>MEEASSISRYLYTFIVLFIIWLFLTASLDPQELTIGALFSAIAALFTYEIFTTRGLANLHPKRVLYFIAYIPYFLWAMIMANLDVAYRVLHPKRPINPGIVECKTTLTNNVGKMALANSITLTPGTITLDVDGDKYFIHWIDVKDSSVEGASEHITKPFEKFLRVIFE[2x];>[2x]MIGVNIYLLLIGVATLLSMYRVFRGPTTVDRLVAVDIMTTITVGLMVLFALYYRRIIFLDVALVYAILSFAGVIAFARYLEGGL;>[2x]MSVLSLIGELLVLFGTVFYLLSTLGLIRMPDVYNRMQTATKSATLGSLGVIIGTGIWALGEGFSVAWLTKAIVIAAFLLLTNPISAHALIRAAYKSGIPLWEGSVVDKYKEHLERKKKEEGEQE;>MNCIVCIEYIIVALMIISAILAVEWRDLLASTVGMAAVSLFASILFFFLQAPDVAMTEAAIGAALSAAVFIFAIKRTYRYETEEEEKLGWWVRW[2x];>[2x]MLKRVLAILTILVIGYWLAQGLADVPFGQDKMVVGKYYLEHVKEETGAVNAVTAVVVNYRGLDTLGEVTVLFIASTGVAALLWKKKRERTAKTEGSVVLTTGARLLFPFIALFGMYIFIHGHLTPGGGFPGGATIATAFLLMYLAFTIYEIPHRGFEVTEGLAGMGYVITGLIGLAIGGYFLFDWIWQTWGWGHENIGRLFSGGFIPIIYTLIGIKVGTELSGIVDNMLKEEVKE;>MISSYYFGAISLILIGLYAVLVKKNLLKILIGLSIMETGVNLLLISIGYVSGKSAPILSEGVTASNAVDPIPQALVLTAIVIGVATTAMALSVAILLYEKYGTLNIEEIRRLRG[2x];>MSQVAALLIALPLISAFFVPVLKQIGKSLIKPFLVIITLLQTLIASWAFVQVYSTGKPIIIYAGGWKPPIGINLYIGHFAALFILVIAVVSFLMALFNFKAVTVEPIDKYAMLFLLLLLGATGMIATGDIFNLFVFMEITAISAYALTAYNKTGEAAEASMKYIVLGGIGSSFFLVGVALIYGATGTLNMAHLAMLANDINPTVVQVGLALIIFGLAVEAELFPLNAWAPDAYQAAPHPITVMFSAFVVKAGLYAMARILYLFKDVSGWSSLTKLLIAMATLTVVFAELSALRQKNVKRMIAYSSIGQVGLIALALSLGTQEGVSAGVFHMLNHAIVKTMMFMAIGYVGITLGGTMIENFEGLGKRMPLTSLSLTIGGIATVGVPLFNVFWSKLRIILAAAHEGNLWPVALVLFASVVEAVYYFRLIHTMWFKGKSGERIPEGAIAIVLLLLAMLIIVIGVYPTPFWNLVTKAGSDIVEVSKYVANVLPGVKL[2x];>MVDWRLFEPLFNWARKKSLWIVAFCTGCGGIEMPPLMTARYDLERFGIMPDPSPRQYDLFLITGYVTPKTLKRIIITYEMAPDPKYVLAHGSCPINGGIYWDAYNAIKQLDKYIPVDVYIAGCMPRPEAVMDGIKKLMEMIENGEADGWKRYKENYEWYRKNQDELLGEGWREKEARKWIPWLMDKRKEVKE[2x];>[2x]MTWEKGEEIVKQILEKAPYAEGKVRRERRLEFRVPADKIRDFLRIMKESNFPLMLQITAVDWPKEGEIELVYHLINVELGTHAMVKTRIPRDLDKARMPTVKDIYPAAETYERDVHDFFGVYFEGNEKMEMPWILDDPERGLYPHRKDFDMLAYVKKKYKILDRFDEDKDKYVI;>[2x]MVSQEELIREARQNGMELYPIDKDTYELFFGPQHMATENFSIILKMDGNRVVKAIANPGFLHRGFEKLAEYRPWYTNIALLLRICVPEPDVPEAIYSMAVDEIIGWEVPERAQWIRTLVLEMARVTAYLFWIMGLSFKLGVYTAGQWAAAYRERFMALFEQLTGARVYHIYTIPGGVRRDIPGDKWLRQVRDTVEYLKDKLKDFDNVLFENYITYKRLEGIGVMDKKFALEEGVTGPNLRATGVAYDVRKSDPYLLYPELDFEIPVLKEGDALARVLVRRYELEQDLYIIEQLLDMGPPSGPYKVQDPKLKNLPRFKVPPGEAFAHVEATKGDFGAYVVSDGGHKPYRVHIRGPSIAHGVRVLEQLLVGARLADVPAILMSLDNCPPDIDR;>[2x]MIGVFLRALLIIIYATFVGFIFMGIIRKVTARIHRRIGPPIYQPIIDTLKFFGKKENITHGLIYDFGIIYAVGATILALMFIPLGPISVLRAYGDLILVTFLLEIPMLGIMFAAMSSGNPYAGIGAQRALLTLLAIQVPLGLAIIAVAEYYGTFSTYEIVMAQQKMGWSIFHLPLLLAAIAYDIVLQAMFGKEPFDIMIAPGEISLGPMVEFGGKHMGMLQIQHAMALFAETLFFSNIFLGGGVVTAFGSPLLNTLASLAVLLVKQIAVLLIAIFVGAIFPRFTIDQAAKFYWKWPTIIAAIGAIMASL;>MEEVTFRIAPEEKVKKKPSFLKPWFGLKYLFKKPVTIKIP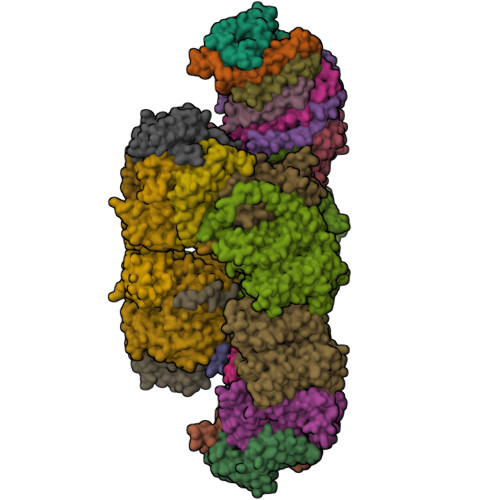YEFIEPAPRYRGFHTLDWKKCIGCNMCGQICPARAIEMTWIEGEKRPHPKIDYGRCTFCQFCVDVCPTGALGFIETYMLTTTWREEELLLYDWVPIEPEKFKEIQEKFKDYKFPVEKIEFNKETKEVTYYLRDGTTFKFKILGYGLKPPVKPQPTTKQQEEEKKESGQ[2x];>MNELPIILLSPLIGGALAWLIRVKGIREAIGVVSSAIPLYFLIKLYPALEGEPIRYSLNVGGFELTLALSHISWIFAMIAAVVGLSAVLGLVSTAKDSNEWLFALMSLAGALGVFLANDFVVFFLSWEIMTFASFMMVFKYNRHASLKYFVLSIAGAYAMLLAIGIIYAKTGSLSFPEISAIFRQDAMMGMMGGGGVFTKTETLLIYALFLVAFGVKAGMFPLHVWAPDAYSETNQSYTAMFSGVLSKTGVYGFFLLYLLMYGKLAITLGNVRSAPTFGYIIAFLGGLTIMVGGILAALQEDIRKLFAYSSISQIGYILIGLGIGTPLGIAAATYHAISHALFKGLFFLIVATIIYRTGKTEFKDYGGLAEKMPITFAMAFVAILSLAGIPPMAGFASKWLIFEAVISRNLPILGAMVFFGSAIGFVYLIRFTYAVWFGQRPSDLEDVKDAPLPLAIGMGILAILNVIFGVAPGLVARELNKLFSNPPIGGTIWELDLGFGRYNGLLLSIWLVIGLIIAAILYFMGAGVRKVPVTDTYQSGNPVTMEYNLTIRRNFFLPLKEAMAFWLKMSFDRLYHDIWKAIEELADLARSYVYNGNIQAYAWYLAIILLILVAMGV[2x]N-[(1S,2R,5R,6R)-2-AMINO-5,6-DIHYDROXY-4-(HYDROXYMETHYL)CYCLOHEX-3-EN-1-YL]ACETAMIDE 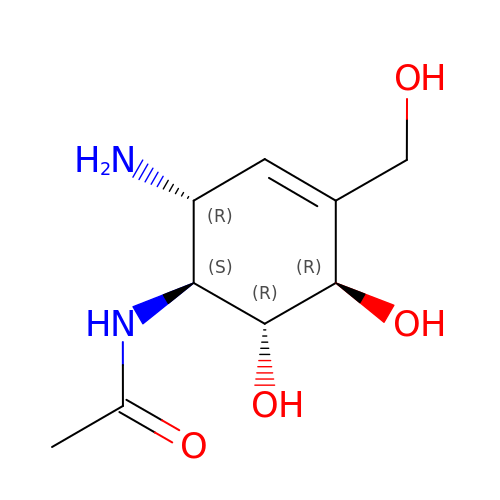| C9 H16 N2 O4 | WWUMIYBLWZAJTD-BZNPZCIMSA-N>SDRPLSVHLNLGQKGNRKTSCPIKINQFEGHFMKLQADSNYLLSKEYEELKDVGRNQSCDIALLPENRGKNRYNNILPYDATRVKLSNVDDDPCSDYINASYIPGNNFRREYIVTQGPLPGTKDDFWKMVWEQNVHNIVMVTQCVEKGRVKCDHYWPADQDSLYYGDLILQMLSESVLPEWTIREFKICGEEQLDAHRLIRHFHYTVWPDHGVPETTQSLIQFVRTVRDYINRSPGAGPTVVHCSAGVGRTGTFIALDRILQQLDSKDSVDIYGAVHDLRLHRVHMVQT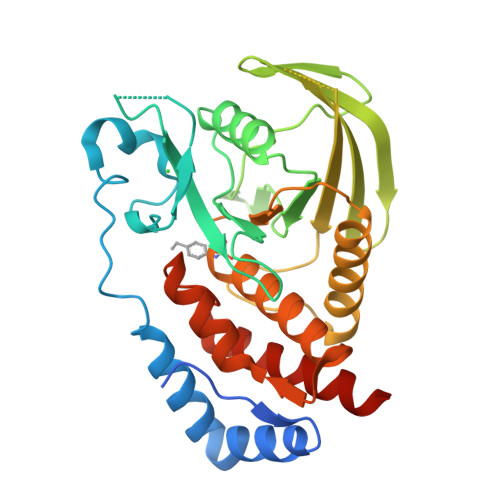ECQYVYLHQCVRDVLRARKLRSEQ[2x]> MPYIEKLELKGFKSYGNKKVVIPFSKGFTAIVGANGSGKSNIGDAILFVLGGLSAKAMRASRISDLIFAGSKNEPPAKYAEVAIYFNNEDRGFPIDEDEVVIRRRVYPDGRSSYWLNGRRATRSEILDILTAAMISPDGYNIVLQGD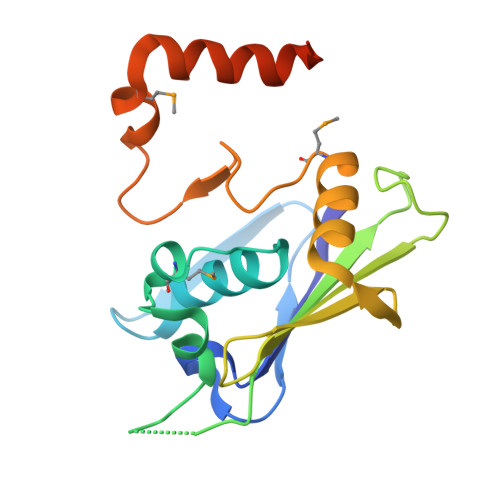ITKFIKMSPLERRLLIDDISGIAEYDSKKEKALEE noscapine | C22 H23 N O7 | 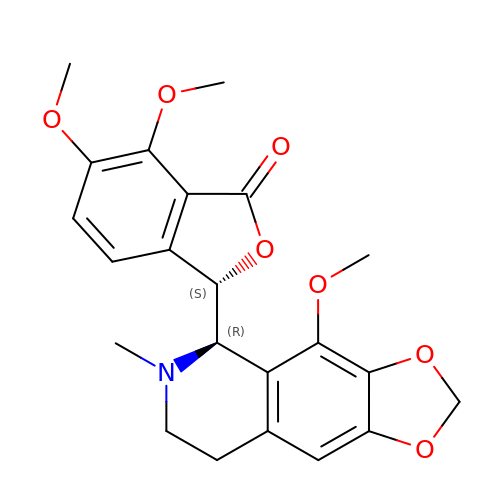AKNNEGZIBPJZJG-MSOLQXFVSA-N>SNAMTRVLYCGDTSLETAAGYLAGLMTSWQWEFDYIPSHVGLDVGELLAKQDLVILSDYPAERMTAQAIDQLVTMV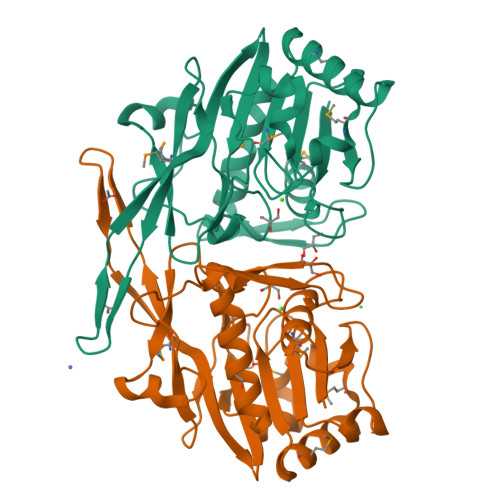KAGCGLVMLGGWESYHGLGGNWDQTLLAEVLPVDIKSADDRINFDQPTLAIPAAINSVSHPILQNLPWEDRPPTIGGLNRIAAKAKAQTLLMARVWRPTFSLEHGKTTWEHADHHPLLVVGEAGTGRVAAFASDVAPHWVGGLVDWGDERVTSQAPGAGAIEVGNLYSQFFRQMLEWVAKSTR[4x]> MGSSHHHHHHSQDPMEIDELTALGGLLHDIGKPVQRAGLYSGDHSTQGARFLRDLAENTGRAEYELLSLFSEFHHKGHMKNDELMIRRIKELSPERFGLTMEDVLNALWIVYEADNLASGEREEGQPQASRPLYSVFNPGKAYPWAELDFEKELPVPGDVFSIRSQDYRELVKRLWEELSKAKLRSDRLLPVLEKYLTFVSSVTSEGNIISLYDHMRMTSAIALAMLRAGCTAEDVRSGRCRKEKRFLLIEGDFSGIQDFIYRVSGKGTLKYLRARSAYLELIGWDVVLEILSRLGLTRANVVFNAGGHFMIIAQNTPDAVKELEEIRAKAVEWLYREFESDLYLAIEWEPVSGREFGREGGKNLFAEARKRLKHKLTVRKLKRFGEIKGLFEHGHTERLAECPVCGRELPEGKLEPSASDPETKVCPTCNRLVSLGGNLPKLLGFGRTAKNDAGVLVEGPFSGFVPYLQGGRPVGEQILVKNTLNPGEIPESAQFVPYFVADYFKKDPKGGVATFEELSMASTGTRRLGVMKGDVDRLGEFFSSMDSPSKLATASRFMDYFFKGYIGAIIEGKFGYIIGDVPSLRDWPEEPDIVVVYAGGDDFFIVGAWDQIFELAFRVRRAFNAYTGGKLTLSVGLGYFDERTPIYRMADVVSERLDTAKDEGRNRVFVVGRSRPLDGKHKLSYEWNHYEELWRTYAPRIYAGNGRLKGKLESKKGLLWKLLEIRELYVRDPNDVRWAYLTAYLLGRHGLSDLFPELVGIDTKAVERKEPQPVYWVDGVLKIVLMAVRR;> SMAYHQKHGGYGRGGYGRQDRPQVDASRLFGESPDVVGIKKMLEGKGKQWEAIQPYFDNVVREAKNFLEWSPNKRLANAVTVAAYLTSQGLKTNQVRKILDMARTTELKVKRGEGDIKDDLVKMRYLLAYTVGKATGQSKYSLDAFHRILDPMLEVLMGSPKKENFEKFYDFLQAVVAYHKFFGGGD;>SMDRRFYGKIVIKGKIKAVTGLHIGSQRDISEIGGIANPVIKDPHTGLPYIPGSSLKGRLRSLFEILVNSRLGEWREKYPSLANYSPGSCRPDNQENCGKFFNRKINRGWIHVCPDYETALACPVCRLFGASGKESNFPSRIIVRDAFLTKEWEEKWRAGEAITEAKIEVGIDRVTSQANPRTNERVVAGAEFEFEIIYNVENTTHWRDDIKNLLTAMALLEDSYLGGSGSRGYGKVKFIFDSFEFRPLDYYRTGKDEDIVSIDAREKSVSDILSGFDSLFSEVEGKLEAG[2x];> MPKFIAVKLIPKGPFRDIPRADTLFGAIGNAISAIHGQSAVEELVDAFVGGARISSAFPYSGDTYYLP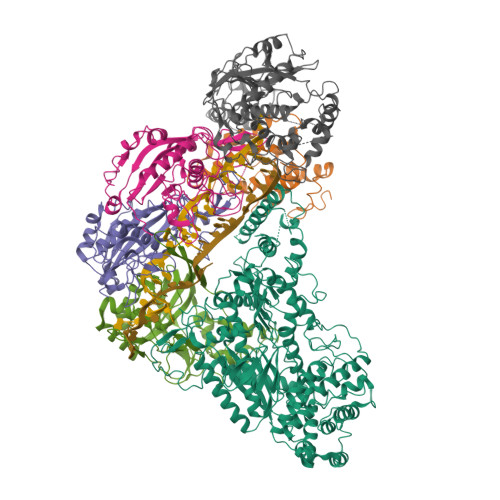KPLSVEPALEGILTGLDEEERYTTAKRLRKAKYLDLKNFELALRLRPFTIPEEIPYARVDVPRVVLDRVTQDSSIYFWEEIRFREKSGVYFLYSGPREVFDGYIAPAMRFLGDTGIGGKSTWGAGLFEVEFHEMKIDAPGSEYSVTLSNALPTKTPVLWRLLRKGGWSFGRRKPRMTFIAEGSIVKNDPGGMERLELGLSHEVYVYGLTFPLGVELPEGLE;> MTERTLKVLSPLHIGTGNELTPVDIYPRENIIHVLDTERLVNDLMNLGVELNEILALLKNPPGDAYIWKGYIEEFHLDPSDYSIYTLKIHGKIGRKSMQIKEFIKLNGRPYIPGSSLKGAIRTAVLYKALKECGDARAVMRVVSKVNGDVARDIGRSEDVLDYYMSFLSRARIDRKRADDLLEAIVFGMEPDRRSKIRYEPKRDPMKALIVRDSKPVGRKHLAVYHVEVIGNPQPIPIWVEAIEPGAATDVEIHVDTEALRLNADYFNGLLWECLKERGEPGEVFEDFLWEAVDEFYTAVMKYETIEVQKFGRYTSQVRSFYASLEDHSGHVLRLGWGSGWLAMTIGLLLVEKGYKWENVRKKLGLGKKPGGSGFSREFPKTRRLADGMPMGWVVLEHHHHHH>CCTCCGGAGG[2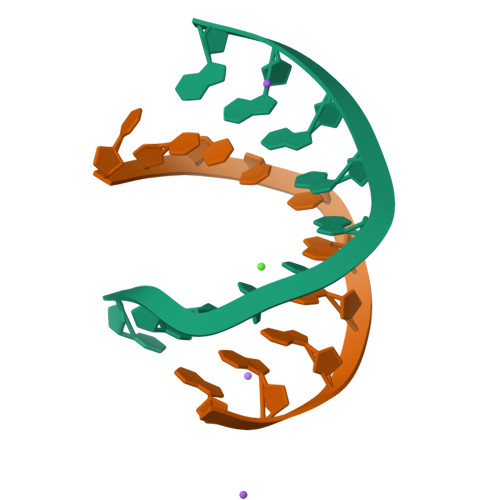x]>ETGGNQNQLLSTLATIRTGKKQVSNCSTNIPLVNDLRFINGINKFIIEDYATHDFSIGHPLNMPSFIPTATSPNGCTRIPSFSLGKTHWCYTHNVINANCKDHTSSNQYISMGILVQTASGYPMFKTLKIQYLSDGLNRKSCSIATVPDGCAMYCYVSTQLETDDYAGSSPPTQKLTLLFYNDTVTERTISPTGLEGNWATLVPGVGSGIYFENKLIFPAYGGVLPNSTLGVKSAREFFRPVNPYNPCSGPQQDLDQRALRSYFPSYFSNRRVQSAFLVCAWNQILVTNCELVVPSNNQTLMGAEGRVLLINNRLLYYQRSTSWWPYELLYEISFTFTNSGQSSVNMSWIPIYSFTRPGSGNCSGENVCPTACVSGVYLDPWPLT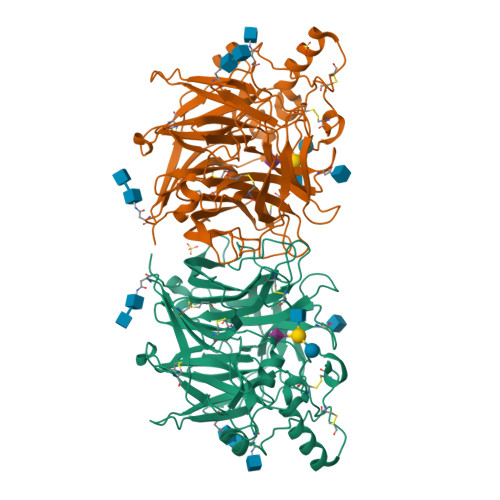PYSHQSGINRNFYFTGALLNSSTTRVNPTLYVSALNNLKVLAPYGNQGLFASYTTTTCFQDTGDASVYCVYIMELASNIVGEFQILPVLTRLTITGTKHHHHHH[2x]Here we elucidate the molecular basis of high-affinity phosphite and hypophosphite acquisition by determining the ligand-binding affinity and structure of the PBPs of phosphite and hypophosphite ABC transporters from environmental microorganisms. We over-produced and purified PBPs of three putative phosphite transporters; PtxB from the globally important marine diazotroph Trichodesmium erythraeum IMS101 (Te_PtxB), PhnD from the oceanic picocyanobacteria Prochlorococcus marinus MIT9301 (Pm_PhnD)35 and PtxB from the soil bacterium Pseudomonas stutzeri WM88 (Ps_PtxB), as well as a PBP from a putative hypophosphite transporter, HtxB, also from P. stutzeri WM88 (HtxB)18. The structures reveal that ligand specificity, measured here by thermophoresis, arises from a combination of steric considerations and the interaction between a ligand P-H hydrogen atom and an aromatic π system in the binding pocket. The structures of two distinct types of phosphite-binding protein and a hypophosphite-binding protein reveal that a P-H…π interaction ensures high-affinity binding of specific ligands, representing a universal mechanism in these PBPs for recognising ligands with a P-H bond.

To determine the structural mechanism of phosphite selectivity we co-crystallised Te_PtxB and Pm_PhnD with phosphite resulting in high-resolution structures (1.95 and 1.46 Å respectively) of the closed, ligand-bound complexes. In the closed form, the amino acids that form the walls of the binding pocket pack tightly against the phosphite moiety and a single water molecule that is also buried in the binding pocket. Each oxygen atom of the phosphite contributes to an extensive hydrogen bonding network to the main chain and side chains of a cluster of conserved residues from lobe 2 (Te_PtxB; Y55, Y100, S130, T131, S132 and H160; Pm_PhnD; Y46, S126, T127, S128, H158 and D205, Figs. 1d, e and 2e, f). In Te_PtxB, it is not possible to determine the protonation state of the phosphite from the pattern of hydrogen bonding, but given the pH of the crystallisation experiment (pH 4.2), it is also likely that the mono-anionic form of phosphite is bound (phosphite pKa 1.5, 6.739). Both proteins contain a conserved histidine as one of the phosphite ligands (Te_PtxB; H160 and Pm_PhnD; H158), which could help stabilise the negative charge on the phosphite. In Pm_PhnD the equivalent interaction is made to a buried water molecule outside of the binding pocket and the hydrogen bonding network around this water molecule is not sufficient to determine the charge on the histidine. In both structures, the hydrogen atom at the R1 position of the phosphite points towards lobe 1, packing against the face of the aromatic ring of a tyrosine residue (Te_PtxB; Y208, Pm_PhnD; Y206).

> MNPKVLKVGAIPDQNQDVLDKRFNLFSKELSKQLDVEVKYIPVINYIAAVTGFRTKDLDLVWFGGLSGVQARLQTPNSIVIAQRDIDKEFKSVFVVNKNLELNSISNIKGLKKLKNLRFTFGSENSTSGRLMPEYFLNQAGVEIKHFKGKKAGFSGSHDATIALVNSGAFDAGALNKQVWENNLKNNPKRTSNLELFWITPEYVDYHWVAQGDLENRFGEGFTKELKSVILNLDIKQKSHKQILDMFNAKRFIKAESKQYKNIEEIGRKLNKIRLEHHHHHH> NNVGPIIRAGDLVEPVIETAEIDNPGKEITVEDRRAYVRIAAEGELILTRKTLEEQLGRPFNMQ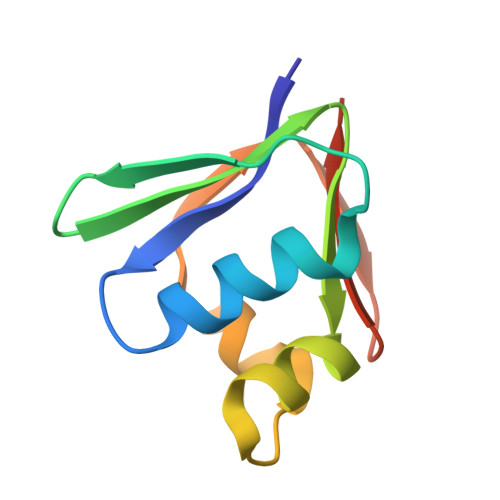ELEINLASFAGQIQADEDQIRFYFDKTM;> NNVGPIIRGDLVVEPVIETAEIDNPGKEITVEDRRAYVRIAAEGELILTRKTLEEQLGRPFNMQELEINLASFAGQIQADEDQIRFYFDKTM Alcohol dehydrogenases (ADHs), also known as ketoreductases (KREDs), are of great industrial interest primarily due to their ability to perform an asymmetric reduction of aldehydes and ketones. Switching the cofactor preference of NADP-dependent enzymes to NAD is of particular interest due to the lower cost and higher stability of NAD, and the higher efficiency of cell-free NAD recycling systems, for which low-cost co-substrates are available. We crystallized CBADHS and TBADHS1 in order to elucidate the structural basis for the observed reversal of cofactor preference. In both cases, the size of the cofactor-binding pocket is reduced due to the substitution of residues 198 and 199 by others with bulkier side chains, which sterically prevents the binding of the 2′ phosphate of NADP.

We performed full combinatorial saturation mutagenesis of residues G198, S199, R200 and Y218 of TBADH to generate a library (TBADHLib) of 16.8 million unique genetic variants. A similar selection procedure as for CBADH was followed but using the ALPS strain, and two different variants were identified, TBADHS1 and TBADHS2. TBADHS1 had substitutions G198S, S199K, R200P, and Y218V. When the enzymatic activity was assayed, TBADHS1 could oxidize isopropanol only with NAD+, certifying the reversal of cofactor preference. The kcat of TBADHS1 for the oxidation of isopropanol with NAD+ was 112 ± 5.7 min−1, 4.5 times lower than the kcat of TBADHWT for the same reaction with NADP+. However, the Km of TBADHS1 for isopropanol was 3.74 ± 0.54 mM, a 32-fold decrease (improvement) compared to the Km of TBADHWT for isopropanol in the presence of NADP+. Overall, the catalytic efficiency (kcat/Km) of TBADHS1 for the oxidation of isopropanol (kcat/Km = 496.67 M−1 s−1) was more than seven times greater than that of TBADHWT with NADP+ (kcat/Km = 70 M−1 s−1). The resulting maps showed clear density for NAD+ in the case of CBADHS, but only partial occupancy for TBADHS1.

>[4x]HMMKGFAMLSIGKVGWIEKEKPAPGPFDAIVRPLAVAPCTSDIHTVFEGAIGERHNMILGHEAVGEVVEVGSEVKDFKPGDRVVVPAITPDWRTSEVQRGYHQHSGGMLAGWKFSNVKDGVFGEFFHVNDADMNLAHLPKEIPLEAAVMIPDMMTTGFHGAELADIELGATVAVLGIGPVGLMAVAGAKLRGAGRIIAVSKPPVCVDAAKYYGATDIVNVKDGPIESQIMNLTEGKGVDAAIIAGGNADIMATAVKIVKPGGTIANVNYFGEGEVLPVPRLEWGCGMAHKTIKGGLCPGGRLRMERLIDLVFYKRVDPSKLVTHVFRGFDNIEKAFMLMKDKPKDLIKPVVILA> EAPYASLTEIEHLVQSVCKSYRETCQLRLEDLLRQRSNIFSREEVTGYQRKSMWEMWERCAHHLTEAIQYVVEFAKRLSGFMELCQNDQIVLLKAGAMEVVLVRMCRAYNADNRTVFFEGKYGGMELFRALGCSELISSIFDFSHSLSALHFSEDEIALYTALVLINAHRPGLQEKRKVEQLQYNLELAFHHHLCKTHRQSI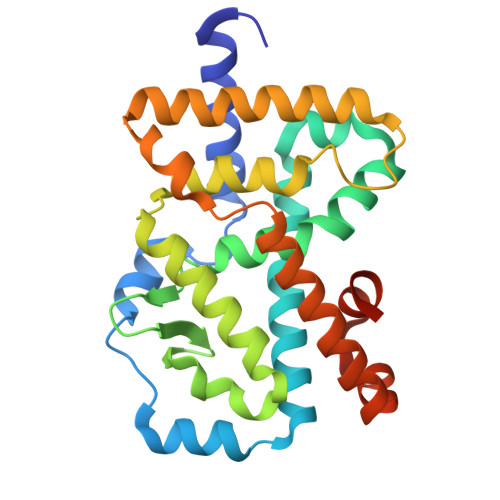LAKLPPKGKLRSLCSQHVERLQIFQHLHPIVVQAAFPPLYKELFSTETESPVGLSK>[55x]MAQVINTNSLSLITQNNINKNQSALSSSIERLSSGLRINSAKDDAAGQAIANRFTSNIKGLTQAARNANDGISVAQTTEGALSEINNNLQRVRELTVQATTGTNSESDLSSIQDEIKSRLDEIDRVSGQTQF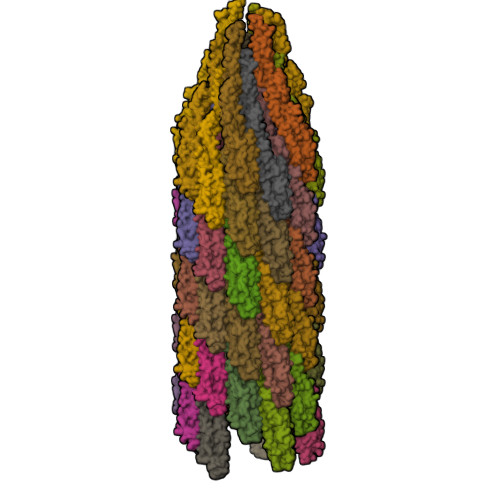NGVNVLAKNGSMKIQVGANDNQTITIDLKQIDAKTLGLDGFSVKNNDTVTTSAPVTAFGATTTNNIKLTGITLSTEAATDTGGTNPASIEGVYTDNGNDYYAKITGGDNDGKYYAVTVANDGTVTMATGATANATVTDANTTKATTITSGGTPVQIDNTAGSATANLGAVSLVKLQDSKGNDTDTYALKDTNGNLYAADVNETTGAVSVKTITYTDSSGAASSPTAVKLGGDDGKTEVVDIDGKTYDSADLNGGNLQTGLTAGGEALTAVANGKTTDPLKALDDAIASVDKFRSSLGAVQNRLDSAVTNLNNTTTNLSEAQSRIQDADYATEVSNMSKAQIIQQAGNSVLAKANQVPQQVLSLLQG The X-linked neuroligin 3 (NLGN3) gene encodes the postsynaptic adhesion molecule NLGN3, which interacts with presynaptic neurexins (NRXNs) to organize synaptogenesis. Here, we identified a non-canonical synapse-organizing interaction between NLGN3 and PTPδ splice variants lacking the meB peptide, which competed with NRXNs by steric hindrance. To elucidate the structural mechanism of the NLGN3–PTPδ-meB(–) interaction, we determined the crystal structures of mouse apo-NLGN3 ECD (residues 35–684) at 2.76 Å resolution and NLGN3 ECD in complex with PTPδA3B– Ig1–Fn1 at 3.85 Å resolution.

The electron densities corresponding to residues 148–173 and 555–567 were invisible, likely owing to the structural disorder. The first disordered region contains a 19-residue insertion at SS-A. The asymmetric unit of the apo-NLGN3 crystal contains two NLGN3 molecules, which form a dimer. The molar mass of the recombinant mouse NLGN3 ECD determined by size-exclusion chromatography coupled with multiangle light scattering (SEC-MALS) analysis is 160 kDa, which corresponds to the mouse NLGN3 ECD dimer. All reported NLGN dimer structures, including our NLGN3 structure, exhibit a similar dimerization interface, where two helices from each protomer form a four-helix bundle. The C-terminal tail of NLGN3 ECD is disordered in the apo-NLGN3 ECD structure, suggesting that it undergoes a disorder-to-order transition upon binding to PTPδ. Arg448 in mouse NLGN3, equivalent to Arg451 in human NLGN3, is located in the helix next to the dimer interface. The side chain of Arg448 faces the protein core and forms a stacking interaction with Trp495. The R/C mutation seems to affect this local structure in close proximity to the dimer interface. Structurally, the R/C mutation may affect the stability and dimeric assembly of NLGN3.

>[2x]APAPTVNTHFGKLRGARVPLPSEILGPVDQYLGVPYAAPPIGEKRFLPPEPPPSWSGIRNATHFPPVCPQNIHTAVPEVMLPVWFTANLDIVATYIQEPNEDCLYLNVYVPTEDGSGAKKQGEDLADNDGDEDEDIRDSGAKPVMVYIHGGSYMEGTGNMIDGSVLASYGNVIVITLNYRVGVLGFLSTGDQAAKGNYGLLDQIQALRWVSENIAFFGGDPRRITVFGSGIGASCVSLLTLSHHSEGLFQRAIIQSGSALSSWAVNYQPVKYTSLLADKVGCNVLDTVDMVDCLRQKSAKELVEQDIQPARYHVAFGPVIDGDVIPDDPEILMEQGEFLNYDIMLGVNQGEGLKFVEGVVDPEDGVSGTDFDYSVSNFVDNLYGYPEGKDTLRETIKFMYTDWADRDNPETRRKTLVALFTDHQWVEPSVVTADLHARYGSPTYFYAFYHHCQSLMKPAWSDAAHGDEVPYVFGVPMVGPTDLFPCNFSKNDVMLSAVVMTYWTNFAKTGDPNKPVPQDTKFIHTKANRFEEVAWSKYNPRDQLYLHIGLKPRVRDHYRATKVAFWKHLVPHLYNLHDMFHYTSTTTKVPPPDTTHSSHITRRPNGKTWSTKRPAISPAYSNENAPGSWNGDQDAGPLLVENPRDYSTEHHHHHH D-cysteine (D-Cys) moieties are found in firefly luciferin, semisynthetic cephalosporin MT141 and malformin A. D-cysteine desulfhydrase (DCyD) is suggested to take part in the catabolic degradation of D-Cys and D-Cys-containing toxic compounds. The polypeptide fold of StDCyD is similar to those of other fold type II PLP-dependent enzymes and consists of a small domain (residues 48–161) and a large domain (residues 1–47 and 162–328). As in other PLP-dependent fold type II enzymes, the active site is situated in a large crevice between the two domains. StDCyD is specific for D-Cys and βCDA, and shows no activity with ACC, although it shares significant sequence identity with ACCDs.

D-Ser, although analogous to D-Cys, is a poor substrate. Hence, the structures of StDCyD cocrystallized with D- and L-Ser were determined. In these structures, electron density was observed near the active site into which the respective ligand could be fitted. However, the internal aldimine was not disrupted. Presence of non-covalently attached D- and L-Ser at the active site of the structures of these complexes suggests that the formation of external aldimine might be the slowest step in the catalytic reaction for these two substrates. Comparison of these two liganded forms reveals that the enantiomers are oriented with their Cα protons pointing in nearly opposite directions. The proton at the Cα of D-Ser is oriented towards the hydroxyl of Tyr287. Therefore, it is reasonable to suggest that the catalytic reaction with D-Ser is initiated by the abstraction of the Cα proton by Tyr287. This is consistent with the observation that Y287F is completely inactive. D- and L-Ser bind non-covalently at the active of StDCyD without forming external aldimines.

>[4x]MRGSHHHHHHGMASMPLHHLTRFPRLEFIGAPTPLEYLPRLSDYLGREIYIKRDDVTPIAMGGNKLRKLEFLVADALREGADTLITAGAIQSNHVRQTAAVAAKLGLHCVALLENPIGTTAENYLTNGNRLLLDLFNTQIEMCDALTDPDAQLQTLATRIEAQGFRPYVIPVGGSSALGAMGYVESALEIAQQCEEVVGLSSVVVASGSAGTHAGLAVGLEHLMPDVELIGVTVSRSVAEQKPKVIALQQAIAGQLALTATADIHLWDDYFAPGYGVPNDAGMEAVKLLASLEGVLLDPVYTGKAMAGLIDGISQKRFNDDGPILFIHTGGAPALFAYHPHVTYPE> TTGH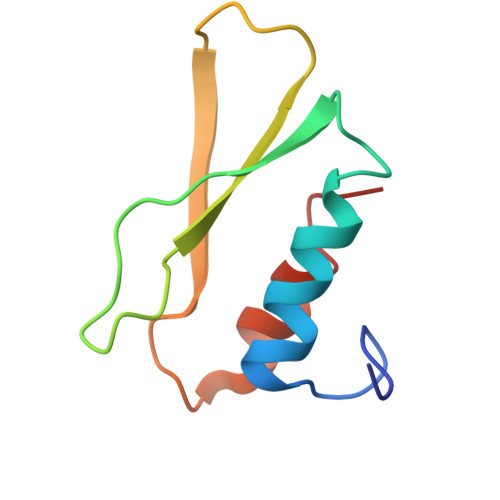SYEKYNNWETIEAWTEQVASENPDLISRSAIGTTFLGNTIYLLKVGKPGSNKPAVFMDCGFHAREWISPAFCQWFVRE> MAKPLTDQEKRRQISIRGIVGVENVAELKKSFNRHLHFTLVKDRNVATTRDYYFAL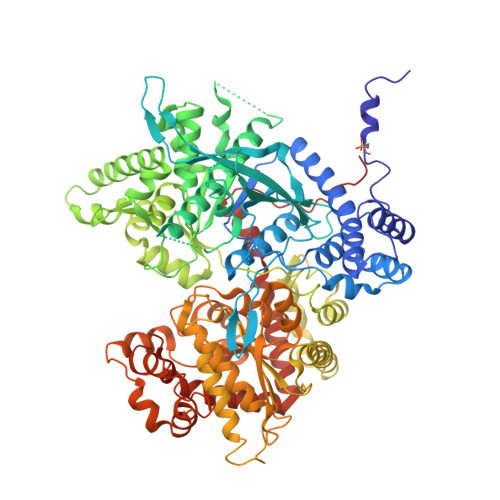AHTVRDHLVGRWIRTQQHYYDKCPKRVYYLSLEFYMGRTLQNTMINLGLQNACDEAIYQLGLDIEELEEIEEDAGLGNGGLGRLAACFLDSMATLGLAAYGYGIRYEYGIFNQKIRDGWQVEEADDWLRYGNPWEKSRPEFMLPVHFYGKVEHTNTGTKWIDTQVVLALPYDTPVPGYMNNTVNTMRLWSARAPNDFNLRDFNVGDYIQAVLDRNLAENISRVLYPNDNFFEGKELRLKQEYFVVAATLQDIIRRFKASKFGSTRGAGTVFDAFPDQVAIQLNDTHPALAIPELMRIFVDIEKLPWSKAWELTQKTFAYTNHTVLPEALERWPVDLVEKLLPRHLEIIYEINQKHLDRIVALFPKDVDRLRRMSLIEEEGSKRINMAHLCIVGSHAVNGVAKIHSDIVKTKVFKDFSELEPDKFQNKTNGITPRRWLLLCNPGLAELIAEKIGEDYVKDLSQLTKLHSFLGDDVFLRELAKVKQENKLKFSQFLETEYKVKINPSSMFDVQVKRIHEYKRQLLNCLHVITMYNRIKKDPKKLFVPRTVIIGGKAAPGYHMAKMIIKLITSVADVVNNDPMVGSKLKVIFLENYRVSLAEKVIPATDLSEQISTAGTEASGTGNMKFMLNGALTIGTMDGANVEMAEEAGEENLFIFGMRIDDVAALDKKGYEAKEYYEALPELKLVIDQIDNGFFSPKQPDLFKDIINMLFYHDRFKVFADYEAYVKCQDKVSQLYMNPKAWNTMVLKNIAASGKFSSDRTIKEYAQNIWNVEPSDLKISLSNESNKVNGN> MDIAKWVEHARTCYSTQLDTKIKVIGVIGKDYPDHGKGDNINCYLRENVFPVAATEDETCTIRGHFSEDDQILFLVMNGVDDVANIRKCLKSNPKSNYFDAMAESECQQIRMLHFLFISCHFIIIFEQTSRIDLELMRFLKKVNSARIQLRKKINQRLVASDLRDVSFNNRILSSAESEGRMVVPRLLIAFQRNNIRPDVNPGKKLQRELYEKLEKNLDNQFSDILKLYDLIDCGASSLCQLNETIPVVHLLNPKIVKRDIIGEMFEILMADAENTKISGNAGTLPSNNSFVKFLEDNFRSEKNEISLENVIELMNCLQCVLDGDLEE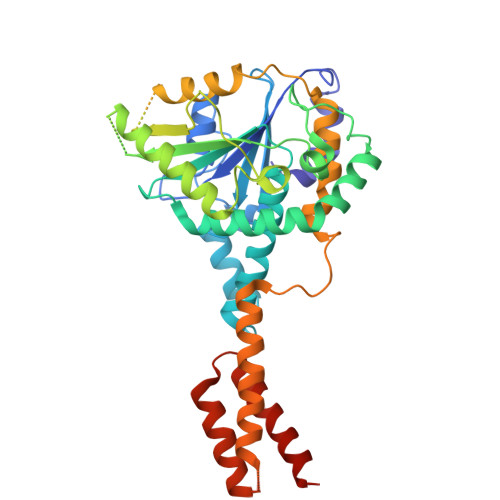KHEKTAIQTFIKRIQNDHMEEARRLYTNAQRPGERRGADRFKDSEKPVKIRSKEEHLMRFNEATHYIDSVVGVNSREALSQLQAQCNEMWQSDMRHHHHHH> IPEYVDWRQKGAVTPVKNQGSCGSCWAFSAVVTIEGIIKIRTGNLNEYSEQELLDCDRRSYGCNGGYPWSAL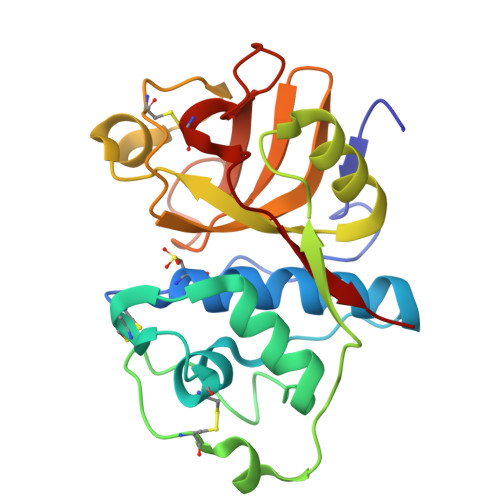QLVAQYGIHYRNTYPYEGVQRYCRSREKGPYAAKTDGVRQVQPYNEGALLYSIANQPVSVVLEAAGKDFQLYRGGIFVGPCGNKVDHAVAAVGYGPNYILIKNSWGTGWGENGYIRIKRGTGNSYGVCGLYTSSFYPVKN Plant vitamin C biosynthetic pathway contains conversion of D-mannose-1-phosphate (Man-1-P) to GDP-D-mannose (GDP-Man), a step catalyzed by the Man-1-P guanylyltransferase which is commonly named GDP-Man pyrophosphorylase (GMPase). Arabidopsis thaliana VTC1 is the first genetically characterized plant GMPase and has unique properties when compared with bacterial and animal homologs. Structures of two GMPases have been reported, which are the crystal structure of GMPase from the hyperthermophilic bacterium Thermotoga maritima (TmGMP) and the cryo-EM structure of human GMPase (GMPPA-GMPPB complex) that is arranged into a dodecamer. These structures show that an oligomer-forming monomer (protomer) of GMPase consists of two domains: an N-terminal Rossmann fold-like domain and a C-terminal left-handed β-helix (LβH) domain. VTC1 dimerizes via its LβH domain and forms a dodecamer in crystal.

The 2.8-Å unliganded structure was solved by molecular replacement using the model based on the cryo-EM structure of the GMPPA-GMPPB complex. In crystal, VTC1 dimerizes in a manner similar to that of GMPPB, with the dimerization interface being solely mediated by the C-terminal LβH domain. Two inter-dimer interfaces were found: the first interface is between catalytic domain and LβH domain, and the second interface results from side-by-side arrangement of two catalytic domains. The first interface could be of biological relevance while the inter-catalytic domain association may be merely due to crystal packing. For structural description, one VTC1 protomer (chain A) was analyzed by the dictionary of secondary structure of proteins (DSSP) algorithm which defined the secondary structural elements. The VTC1 protomer has 7 α-helices, 7 η-helices, and 30 β-strands. The catalytic domain comprises of 14 helical elements and 13 β-strands (β1–β13), and the LβH domain consists of 17 β-strands (β14–β30). The central β-sheet of the catalytic domain is made up by nine strands in the order of β5-β4-β1-β6-β11-β8-β12-β9-β10. Two small β-sheets (β2–β3 and β7–β13) lie near the C-terminal α-helix (α7) of the catalytic domain. The LβH domain has 5 three-β-stranded coils and one two-β-stranded coil.

>MGMKALILVGGFGTRLRPLTLSFPKPLVDFANKPMILHQIEALKAVGVDEVVLAINYQPEVMLNFLKDFETKLEIKITCSQETEPLGTAGPLALARDKLLDGSGEPFFVLNSDVISEYPLKEMLEFHKSHGGEASIMVTKVDEPSKYGVVVMEESTGRVEKFVEKPKLYVGNKINAGIYLLNPSVLDKIELRPTSIEKETFPKIAAAQGLYAMVLPGFWMDIGQPRDYITGLRLYLDSLRKKSPAKLTSGPHIVGNVLVDETATIGEGCLIGPDVAIGPGCIVESGVRLSRCTVMRGVRIKKHACISSSIIGWHSTVGQWARIENMTILGEDVHVSDEIYSNGGVVLPHKEIKSNILKPEIVMKLAAALEHHHHHH[2x]>MNTEALQSKFFSPLQKAMLPPNSFQGKVAFITGGGTGLGKGMTTLLSSLGAQCVIASRKMDVLKATAEQISSQTGNKVHAIQCDVRDPDMVQNTVSELIKVAGHPNIVINNAAGNFISPTERLSPNAWKTITDIVLNGTAFVTLEIGKQLIKAQKGAAFLSITTIYAETGSGFVVPSASAKAGVEAMSKSLAAEWGKYGMRFNVIQPGPIKT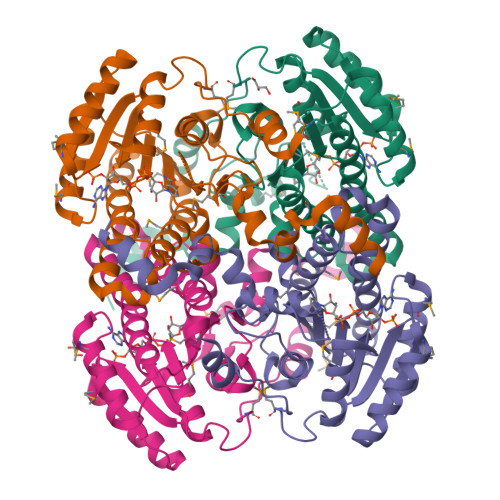KGAFSRLDPTGTFEKEMIGRIPCGRLGTVEELANLAAFLCSDYASWINGAVIKFDGGEEVLISGEFNDLRKVTKEQWDTIEELIRKTKGS[4x]> GGLEKDFLPLYFGWFLTKKSSETLRKAGQVFLEELGNHKAFKKELRHFISGDEPKEKLELVSYFGKRPPGVLHCTTKACDYGKAAGAEEYAQQEVVKRSYGKAFKLSISALFVTPKTAGAQVVLTDQELQLWPSDLDKPSASEGLPPGSRAHVTLGCAADVQPVQTGLDLLDILQQVKGGSQGEAVGELPRGKLYSLGKGRWMLSLTKKMEVKAIFTGYYG

2′,3′-cyclic nucleotide 3′-phosphodiesterase (CNPase) comprises 4% of total myelin protein in the central nervous system (CNS), being the most abundant CNS non-compact myelin protein4. CNPase consists of an N-terminal polynucleotide kinase-like domain10, a catalytic phosphodiesterase domain11, and a membrane-anchored C-terminal tail, which contains a cysteine residue that undergoes isoprenylation. The catalytic domain enables the rapid hydrolysis of nucleoside 2′,3′-cyclic phosphates to nucleoside 2′-phosphates. The CNPase catalytic site, lying in a groove between two lobes, has pseudo two-fold symmetry and contains two apposing His-X-Thr-X (X denotes a hydrophobic residue) motifs, characteristic for 2H phosphoesterases 113537.

In addition to the catalytic His mutants, near-complete catalytic inactivation is evident also in T232A, T311A, F235A, F235L, and Y168A. While recognizing the caveat that the high KM for these mutants makes kcat rather inaccurate, this implies that the π-π stacking between Phe235 and the nucleotide base is not only required for substrate affinity, but it also may define correct substrate docking into a productive binding mode.The enzyme CdaA, which synthesizes an essential second messenger cyclic di-AMP (c-di-AMP) in many pathogenic bacteria, has emerged as a promising candidate for the development of novel antibiotics. Additionally, c-di-AMP regulates the bacterial stringent response, further underscoring its significance. The synthesis of c-di-AMP is mediated by enzymes possessing a diadenylate-cyclase (DAC) domain.

To identify crystals suitable for fragment screening, CdaA enzymes from Streptococcus pneumoniae, Bacillus subtilis and Enterococcus faecium were purified and crystallized. However, suitable crystallization conditions for unliganded LmCdaA could not be identified. Therefore, structurally related CdaA enzymes from S. pneumoniae, B. subtilis and E. faecium were cloned, overexpressed in E. coli, purified, crystallized and evaluated for diffraction quality. Additionally, we report the first crystal structures of apo CdaA from E. faecium (EfCdaA) and S. pneumoniae (SpCdaA), as well as atomic resolution structures of BsCdaA.

>GSHMASMNAPISAEEQMIRAFVKSVEYMSPRKIGALVAIQRVRTLQEYISTGIPLDAKISAELLINIFIPNTPLHDGAVIIKEERIAVTSAYLPLTKNTGISKEFGTRHRAAIGLSEVSDALTFVVSEETGGISITYNGRFKHNLTLDEFETELREILLPKEEVGLSFKERLLGGWKHEKK[6x]During HR, a recombinase binds to single-stranded DNA (ssDNA) and forms a right-handed helical nucleoprotein filament, known as a presynaptic filament, which then searches double-stranded DNA (dsDNA) for homology. Eukaryotic RAD51 and DMC1 both catalyze strand displacement and strand exchange. Interestingly, DMC1 possesses the ability of stabilizing mismatch-containing recombination intermediates (low-fidelity recombinase), whereas the RAD51 lacks the ability to do so (high-fidelity recombinase). RAD51 and DMC1 are members of the RecA family of DNA recombinases and share ~50% amino acid identity and similar biochemical properties.

We next solved the structure of the postsynaptic filaments of DMC1-Q244M with homologous dsDNA (Structure 4, 3.20 Å). Interestingly, the central axis of 2D class averages, where the DNA is located, is different between DMC1 and DMC1-Q244M, and only minor residual DNA maps were detected in the 3D maps of the latter. The results suggest that the Q244M mutant still binds DNA for filament formation but the bound DNA is too flexible to be observed by cryo-EM, likely due to the unfavorable replacement of a polar glutamine with a hydrophobic methionine. On the other hand, the protein structure of Q244M filaments is well resolved and is nearly identical to the structure of wild-type (WT) filaments (the backbone RMSD is 0.80 Å out of 305 Cα atoms), except that the Met244 sidechain points away from the DNA position similar to that in RAD51. Furthermore, due to backbone interactions between Gln244 and Arg242, the sidechain guanidinium group of Arg242 turns away from DNA in Q244M (3.1 Å–4.4 Å). These results suggest that the lineage-specific Gln244 coordinates with the conserved Arg242 to stabilize the backbone of DNA in DMC1, which is weakened in DMC1-Q244M, leading to enhanced DNA dynamics and loss of DNA density. The Loop 1 reciprocal mutants DMC1-Qm and RAD51-Mq changed in opposite directions to 77% and 87%, respectively. As expected, although the 15 nt mismatch substrate is closer to the 15 nt homologous substrate than the 12 nt homologous one in WT DMC1, it is closer to the 12 nt homo in WT RAD51. As shown in the other panels in Fig. 4f, both DMC1-Qm and DMC1-PvGd mutants displayed similar properties to WT RAD51, whereas the reciprocal RAD51 mutants as well as the triple mutant RAD51-MqVpDg behaved similar to WT DMC1.

>[3x]MKEDQVVAEEPGFQDEEESLFQDIDLLQKHGINVADIKKLKSVGICTIKGIQMTTRRALCNVKGLSEAKVDKIKEAANKLIEPGFLTAFEYSEKRKMVFHITTGSQEFDKLLGGGIESMAITEAFGEFRTGKTQLSHTLCVTAQLPGAGGYPGGKIIFIDTENTFRPDRLRDIADRFNVDHDAVLDNVLYARAYTSEHQMELLDYVAAKFHEEAGIFKLLIIDSIMALFRVDFSGRGELAERQMKLAQMLSRLQKISEEYNVAVFVTNQMTADPGATMTFQADPKKPIGGHILAHASTTRISLRKGRGELRIAKIYDSPEMPENEATFAITAGGIGDAKE> AQHPPYCRNQPGKCQ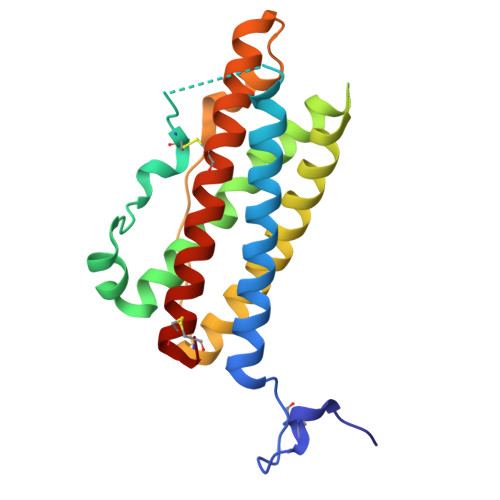IPLQSLFDRATTVANYNSKLAGEMVNRFDEQYGQGINSESKVINCHTSSITTPNSKAEAINTEDKILFKLVISLLHSWDEPLHHAVTELANSKGTSPALLTKAQEIKEKAKVLVDGVEVIQKRIHPGEKNEPYPVWSEQSSLTSQDENVRRVAFYRLFHCLHRDSSKIYTYLRILKCRLTSCET> MKKESINTSGPDNTKSSISDEIEISNEISWTALSGVISAANNADGRLEVFGVGTNNAVWHNWQTVPNTGSSWSGWHSLNEGATSKPAVHINSDGRLEVFVRGTDNALWHNWQTVPGAGWSGWQ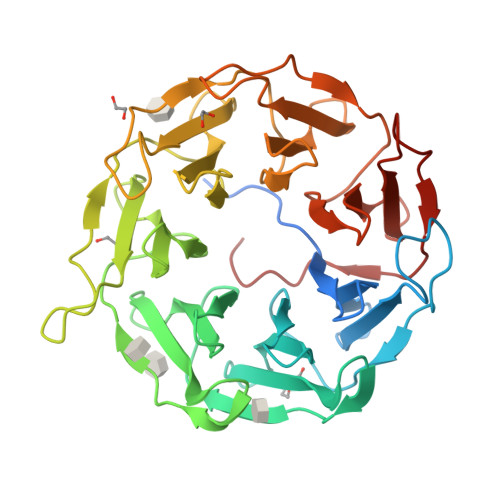SLGGQITSNPVVYINSDGRLEVFARGADNALWHIWQTAPHAGPWSNWQSLNGVLTSDPTVYVNASGRPEVFARSNDYSLWYIKQTASHTYPWTNWQSLSGVITSNPVVISNSDGRLEVFARGSDNALWHIWQVAPNAGWTNWRSLSGIITSDPAVHINADGRLEVFARGPDNALWHIWQTATSDAWSEWTSLSGVITSAPTVAKNSDGWLEVFARGANNALCHIQQTTSSWSTWTSLGGNLIDASAIK>GKAF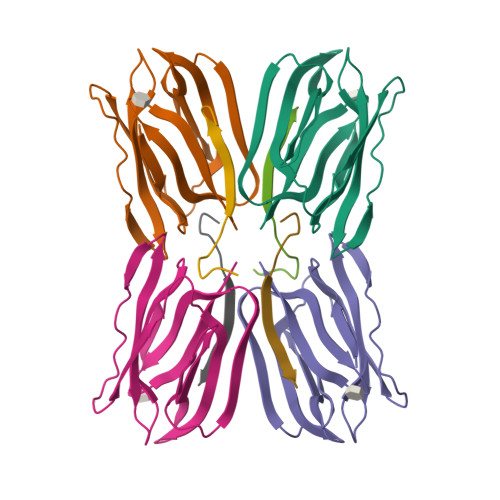DDGAFTGIREINLSYNKETAIGDFQVVYDLNGSPYVGQNHKSFITGFTPVKISLDFPSEYIMEVSGYTGNVSGYVVVRSLTFKTNKKTYGPYGVTSGTPFNLPIENGLIVGFKGSIGYWLDYFSMYLSL[4x];>[4x]NEQSGISQTVIVGPWGAK METHYL 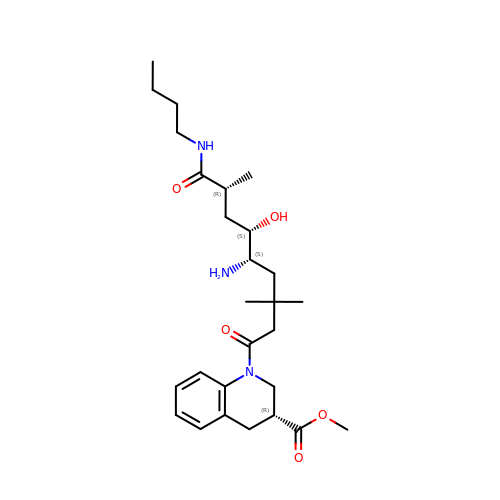(3R)-1-[(5S,6S,8R)-5-AMINO-9-BUTYLAMINO-6-HYDROXY-3,3,8-TRIMETHYL-9-OXO-NONANOYL]-3,4-DIHYDRO-2H-QUINOLINE-3-CARBOXYLATE | C27 H43 N3 O5 | VROPGBJWKDHPPG-WQJYWUQFSA-N2-({4-[(2-amino-4-oxo-4,7-dihydro-3H-pyrrolo[2,3-d]pyrimidin-5-yl)methyl]benzene-1-carbonyl}amino)-4-methoxybenzoic 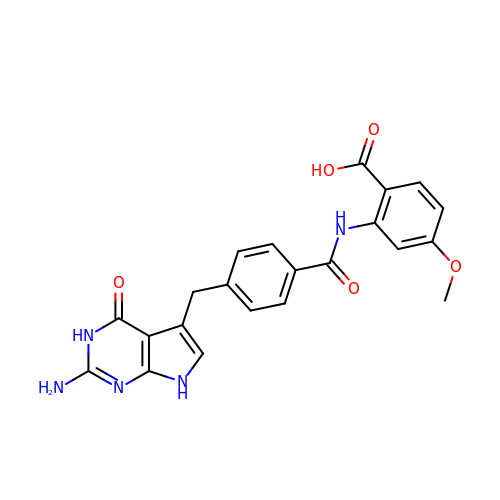acid | C22 H19 N5 O5 | IXAPCYKVLYGBPQ-UHFFFAOYSA-N> EEIIHKL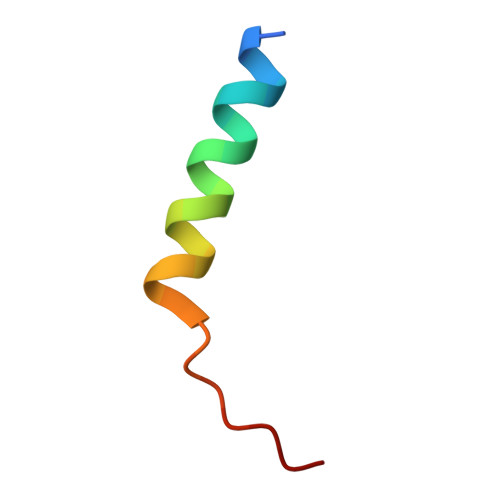AMQLRHIGDNIDHRMVRED> VMGKRYVATPQQSQWEMVVNTPLECQLVHPIPSFGDAVFSSRANKKINLDFELKMRRPMGETRNVSLISMPPPWRPGEHADRITNLKFFKQFDGYVGGQTAWGILSELEKGRYPTFSYQDWQSRDQRIEVALS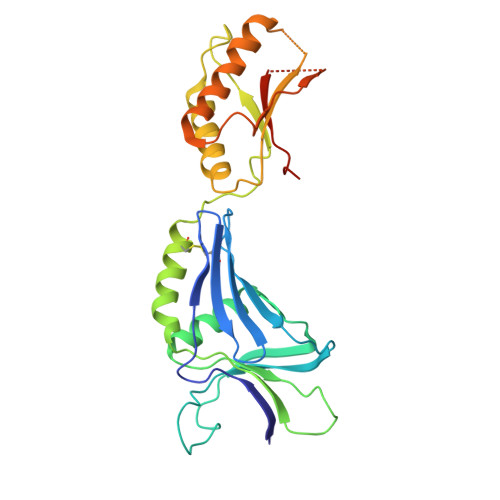SVLFQNKYNAFSDCISNLLKYSFEDIAFTILHYERQGDQLTKASKKRLSQIADYIRHNQDIDLVLVATYTDSTDGKSASQSLSERRAESLRDYFQSLGLPEDRIQVQGYGKRRPIADNGSPIGKDKNRRVVISLGRTQVHHHHHH>[4x]AEGTRGRSSTARCSLFGSDFVNTFDGSMYSFAGYCSYLLAGGCQKRSFSIIGDFQNGKRVSLSVYLGEFFDIHLFVNGTVTQGDQRVSMPYASKGLYLETEAGYYKLSGEAYGFVARIDGSGNFQVLLSDRYFNKTCGLCGNFNIFAEDDFMTQEGTLTSDPYDFANSWALSSGEQWCERASPPSSSCNISSGEMQKGLWEQCQLLKSTSVFARCHPLVDPEPFVALCEKTLCECAGGLECACPALLEYARTCAQEGMVLYGWTDHSACSPVCPAGMEYRQCVSPCARTCQSLHINEMCQERCVDGCSCPEGQLLDEGLCVESTECPCVHSGKRYPPGTSLSRDCNTCICRNSQWICSNEECPGECLVTGQSHFKSFDNRYFTFSGICQYLLARDCQDHSFSIVIETVQCADDRDAVCTRSVTVRLPGLHNSLVKLKHGAGVAMDGQDVQLPLLKGDLRIQHTVTASVRLSYGEDLQMDWDGRGRLLVKLSPVYAGKTCGLCGNYNGNQGDDFLTPSGLAEPRVEDFGNAWKLHGDCQDLQKQHSDPCALNPRMTRFSEEACAVLTSPTFEACHRAVSPLPYLRNCRYDVCSCSDGRECLCGALASYAAACAGRGVRVAWREPGRCELNCPKGQVYLQCGTPCNLTCRSLSYPDEECNEACLEGCFCPPGLYMDERGDCVPKAQCPCYYDGEIFQPEDIFSDHHTMCYCEDGFMHCTMSGVPGSLLPDAVLSSPLSHRSKR;>SLSCRPPMVKLVCPADNLRAEGLECTKTCQNYDLECMSMGCVSGCLCPPGMVRHENRCVALERCPCFHQGKEYAPGETVKIGCNTCVCQDRKWNCTDHVCDATCSTIGMAHYLTFDGLKYLFPGECQYVLVQDYCGSNPGTFRILVGNKGCSHPSVKCKKRVTILVEGGEIELFDGEVNVKRPMKDETHFEVVESGRYIILLLGKALSVVWDRHLSISVVLKQTYQEKVCGLCGNFDGIQNNDLTSSNLQVEEDPVDFGNSWKVSSQCADTRKVPLDSSPATCHNNIMKQTMVDSSCRILTSDVFQDCNKLVDPEPYLDVCIYDTCSCESIGDCACFCDTIAAYAHVCAQHGKVVTWRTATLCPQSCEERNLMENGYECMWRYNSCAPACQVTCQHPEPLACPVQCVEGCHAHCPPGKILDELLQTCVDPEDCPVCEVAGRRFASGKKVTLNPSDPEHCQICHCDVVNLTCEACQEPGGLVVPPHHHHHH[4x]

Von Willebrand factor (VWF) assembly begins in the endoplasmic reticulum of endothelial cells and megakaryocytes where VWF is synthesized as a precursor with multiple domains. The polypeptide including the propeptide and mature VWF chain (proVWF) subsequently forms “tail-to-tail” homodimers through their C-terminal cystine knot (CK) domains. These proVWF dimers are then transported to the Golgi where they assemble into large multimers ‘head-to-head’ through interchain disulfide bonds between D3 domains of two proVWF dimers. Therefore, the disulfide linkages and the cysteines involved in the VWF D′D3 dimer interface remain to be confirmed with the discrepancy mainly on Cys1097 and Cys1099. Here we identified the disulfide linkages from the D′D3 dimer interface through chemical digestion and mass spectrometry and solved the cryo-electron microscopy (cryo-EM) structure of VWF tubules with each repeating unit containing one D′D3 dimer and one D1D2 dimer.

In order to gain further structural information of the D′D3 dimer interface, we purified D′D3 dimers complexed with D1D2 derived from the expression medium of HEK293 cells transfected with expression plasmid of D1D2D′D3-wt or D1D2D′D3-R1136M-E1143M. The tubule-like oligomers of these complexes were analyzed by single-particle cryo-EM. This yielded an electron density map covering two repeating units for D′D3-R1136M-E1143M dimer complexed with D1D2 at 3.3 Å resolution and an electron density map covering one repeating unit for D′D3-wt dimer complexed with D1D2 at 3.4 Å resolution respectively. As the overall configuration of the refined D′D3-wt complex is essentially the same as that of the D′D3-R1136M-E1143M mutant, the structure of the mutant was selected for presentation due to its slightly better resolution. The shape of the repeating unit largely resembles that of MUC2 where a D′D3 dimer is docked in the central hole of the donut-shaped D1D2 dimer8. The electron density near the center covering the D′D3 dimer is unambiguous and a clear density covering the disulfide bonds near the dimeric interface can be observed. The structure showed that D′D3 retained the overall conformation seen in the crystal structure of D′D3 monomer (rmsd of 1.7 Å) but with local conformational rearrangements near the dimeric interface. The connecting loop linking two helices in the D′D3 monomer restrained by the Cys1091–Cys1097 disulfide is anchored in a hydrophobic pocket formed by Phe1100, Met1055, and Val1056 through Ile1094, but in the dimer, it is more flexible with the intramolecular Cys1091–Cys1099 bond and flips over to dock in the same hydrophobic surface pocket of the other D′D3 molecule in a domain swapping-like fashion. This brings two Cys1097 residues in proximity and the subsequent formation of an intermolecular disulfide bond.> CACGTGGACAGGAG;> ACCTCCTGAGGTCGAGC;> TCGCT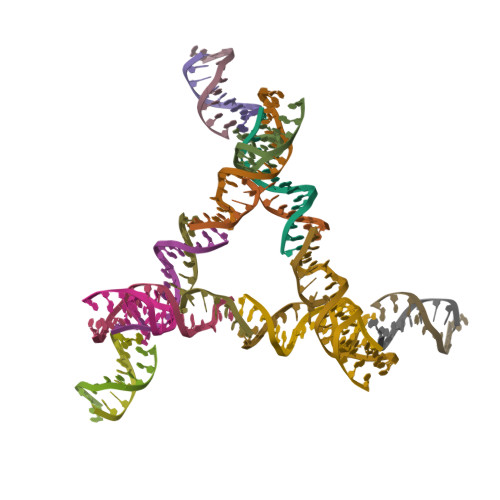CAGCCTGACTCA;> GTGAGTCTCCACGT;> GACTCTGCTA;> GTTAGCAGAG>MITNWMSQTLPSLVGLNTTRLSAASGGTLDRSTGVLPTNPEESWQVYSSAQDSEGRCICTVVAPQQTMCSRDARTKQLRQLLEKVQNMSQSIEVLDRRTQRDLQYVEKMENQMKGLETKFKQVEESHKQHLARQFKAIKAKMDELRPLIPVLEEYKADAKLVLQFKEEVQNLTSVLNELQEEIGAYDYDELQSRVSNLEERLRACMQKLACGKLTGISDPVTVKTSGSRFGSWMTDPLAPEGDNRVWYMDGYHNNRFVREYKSMVDFMNTDNFTSHRLPHPWSGTGQVVYNGSIYFNKFQSHIIIRFDLKTETILKTRSLDYAGYNNMYHYAWGGHSDIDLMVDENGLWAVYATNQNAGNIVISKLDPVSLQILQTWNTSYPKRSAGEAFIICGTLYVTNGYSGGTKVHYAYQTNASTYEYIDIPFQNKYSHISMLDYNPKDRALYAWNNGHQTLYNVTLFHAAAH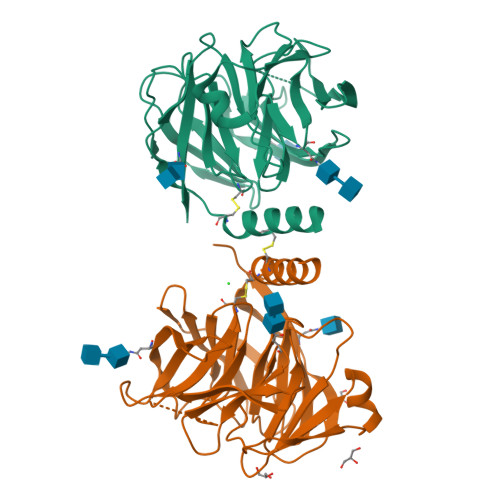HHHHH[2x]>MDAAQQGDTTTILMLPWLGYGHLSAFLELAKSLSRRNFHIYFCSTSVNLDAIKPKLPSSFSDSIQFVELHLPSSPEFPPHLHTTNGLPPTLMPALHQAFSMAAQHFESILQTLAPHLLIYDSLQPWAPRVASSLKIPAINFNTTGVFVISQGLHPIHYPHSKFPFSEFVLHNHWKAMYSTADGASTERTRKRGEAFLYCLHASCSVILINSFRELEGKYMDYLSVLLNKKVVPVGPLVYEPNQDGEDEGYSSIKNWLDKK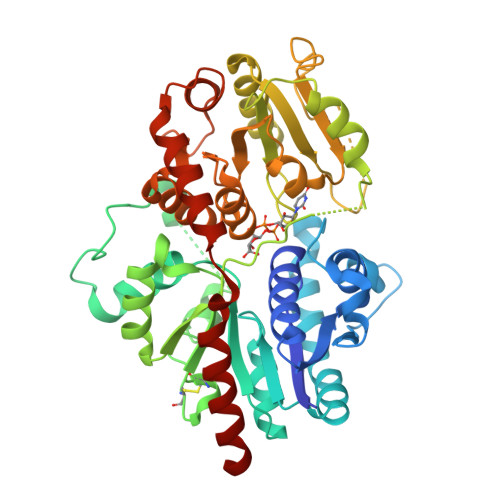EPSSTVFVSFGSEYFPSKEEMEEIAHGLEASEVNFIWVVRFPQGDNTSGIEDALPKGFLERAGERGMVVKGWAPQAKILKHWSTGGFVSHCGWNSVMESMMFGVPIIGVPMHVDQPFNAGLVEEAGVGVEAKRDPDGKIQRDEVAKLIKEVVVEKTREDVRKKAREMSEILRSKGEEKFDEMVAEISLLLKIEHHH[2x]> KKRQWALEDFEIGRPLGKGKFGNVYLAREKQSKFILALKVLFKAQLEKAGVEHQLRREVEIQSHLRHPNILRLYGYFHDATRVYLILEYAPLGTVYRELQKLSKFDEQRTATYITELANALSYCHSKRVIHRDIKPENLLLGSAGELKIADFGWSVHAPSSRRTDLCGTLDYLPPEMIEGRMHDEKVDLWSLGVLCYEFLVGKPPFEANTYQETYKRISRVEFTFPDFVTEGARDLISRLLKHNPS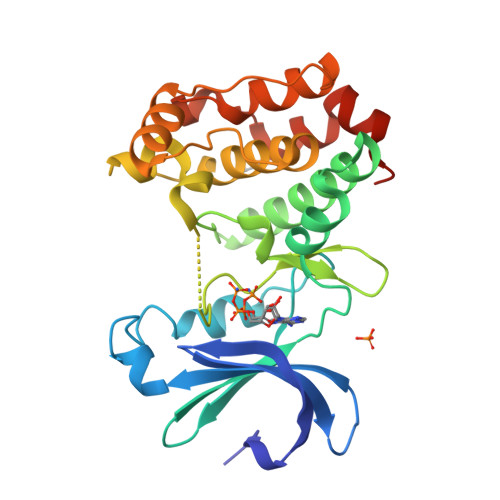QRPMLREVLEHPWITANSSKPSNCQNKES> MATTTPERVMQETMDYHALNAMLNLYDKAGHIQFDKDQQAIDAFFATHVRPHSVTFASQHERLGTLVREGYYDDAVLARYDRAFVLRLFEHAHASGFRFQTFLGAWKFYTSYTLKTFDGKRYLEHFEDRVTMVALTLAQGDETLATQLTDEMLSGRFQPATPTFLNCGKQQRGELVSCFLLRIEDNMESIGRAVNSALQLSKRGGGVAFLLSNLREAGAPIKRIENQSSGVIPVMKMLEDAFSYANQLGARQGAGAVYLHAHHPDILRFLDTKRENADEKIRIKTLSLGVVIPDITFRLAKENAQMALFSPYDIQRRYGKPFGDIAISERYDELIADPHVRKTYINARDFFQTLAEIQFESGYPYIMFEDTVNRANPIAGRINMSNLCSEILQVNSASRYDDNLDYTHIGHDISCNLGSLNIAHVMDSP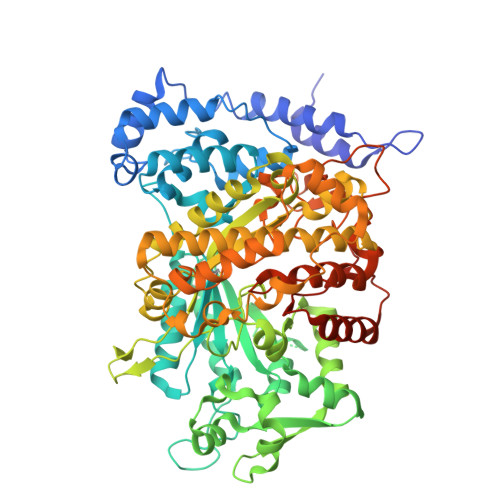DIGRTVETAIRGLTAVSDMSHIRSVPSIAAGNAASHAIGLGQMNLHGYLAREGIAYGSPEALDFTNLYFYTITWHAVHTSMRLARERGKTFAGFAQSRYASGDYFTQYLQDDWQPKTAKVRALFARSGITLPTREMWLKLRDDVMRYGIYNQNLQAVPPTGSISYINHATSSIHPIVAKIEIRKEGKTGRVYYPAPFMTNENLDMYQDAYDIGPEKIIDTYAEATRHVDQGLSLTLFFPDTATTRDINKAQIYAWRKGIKSLYYIRLRQLALEGTEIEGCVSCAL1,5-anhydro-2-deoxy-2-fluoro-D-xylitol | C5 H9 F O3 | 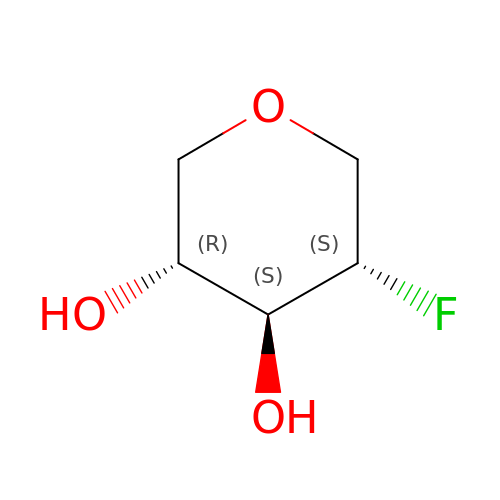YIJTWYXBSRZXRS-VPENINKCSA-N(3~{S},3'~{S},4'~{S},5'~{S})-4'-azanyl-6-chloranyl-3'-(3-chloranyl-2-fluoranyl-phenyl)-1'-[(3-ethoxyphenyl)methyl]-5'-methyl-spiro[1~{H}-indole-3,2'-pyrrolidine]-2-one 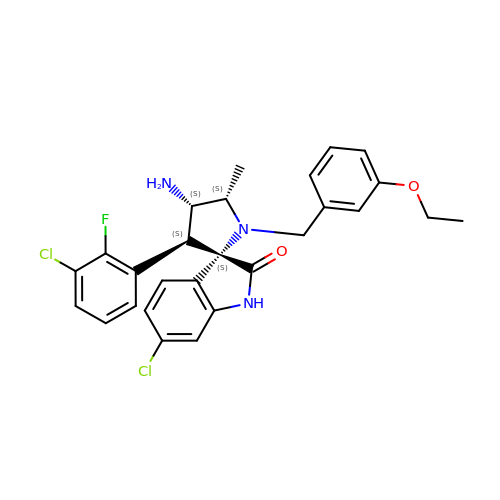| C27 H26 Cl2 F N3 O2 | VTZPRLPCZBTKSH-VFICKSILSA-N> MAHHHHHHNPNYCFAGKTSSISDLKEVPRKNITLIRGLGHGAFGEVYEGQVSGMPNDPSPLQVAVKTLPEVCSEQDELDFLMEALIISKFNHQNIVRCIGVSLQSLPRFILLEFMAGGDLKSFLRETRPRPSQPSSLAMLDLLHVARDIACGCQYLEENHFIHRDIAARNCLLTCPGPGRVAKIGDFGMARDIYRASYYRKGGCAMLPVKWMPPEAFMEGIFTSKTDTWSFGVLLWEIFSLGYMPYPSKSNQEVLEFVTSGGRMDPPKNCPGPVYRIMTQCWQHQPEDRPNFAIILERIEYCTQD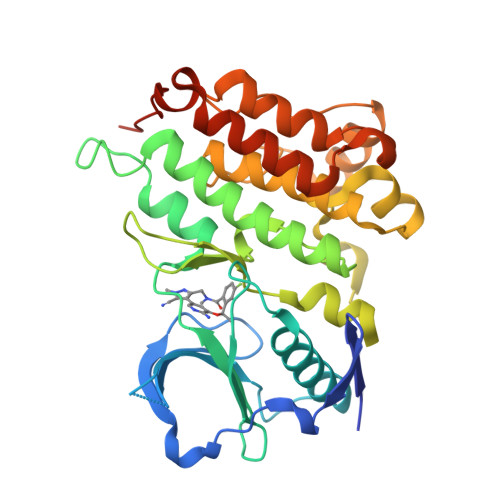PDVINTALPIEYGPLVEEEEKV> GGATACGTAG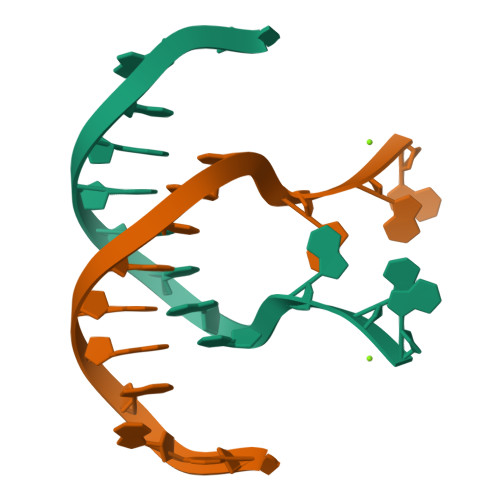GAG> FPTDDDDKIVGGYTCAANSIPYQVSLNSGSHFCGGSLINSQWVVSAAHCYK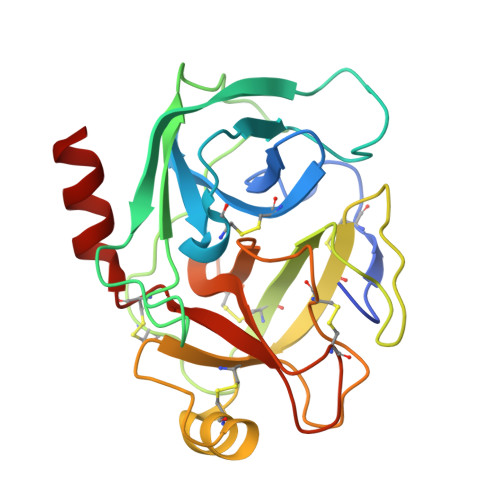SRIQVRLGEHNIDVLEGNEQFINAAKIITHPNFNGNTLDNDIMLIKLSSPATLNSRVATVSLPRSCAAAGTECLISGWGNTKSSGSSYPSLLQCLKAPVLSDSSCKSSYPGQITGNMICVGFLEGGKDSCQGDSGGPVVCNGQLQGIVSWGYGCAQKNKPGVYTKVCNYVNWIQQTIAAN(1R)-3-amino-1-{3-[(4,4-difluorocyclohexyl)methoxy]phenyl}propan-1-ol 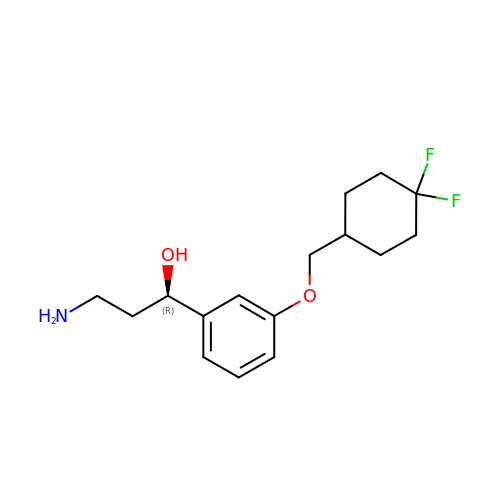| C16 H23 F2 N O2 | SXUQDOSXLJQVRA-OAHLLOKOSA-N> CCGAAT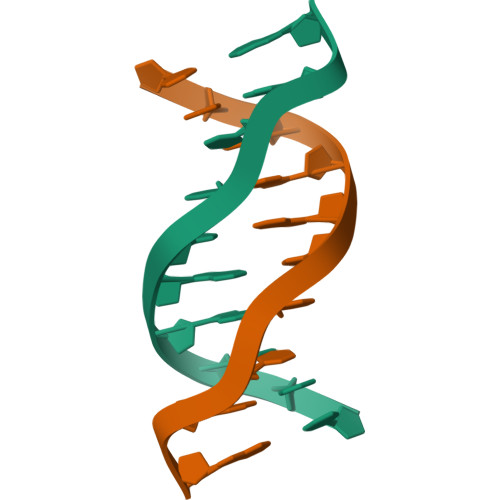TCGG(2~{S})-3-cyclohexyl-2-[[(2~{S})-4-methyl-2-[[oxidanyl(phenylmethoxycarbonylaminomethyl)phosphoryl]amino]pentanoyl]amino]propanoic acid | 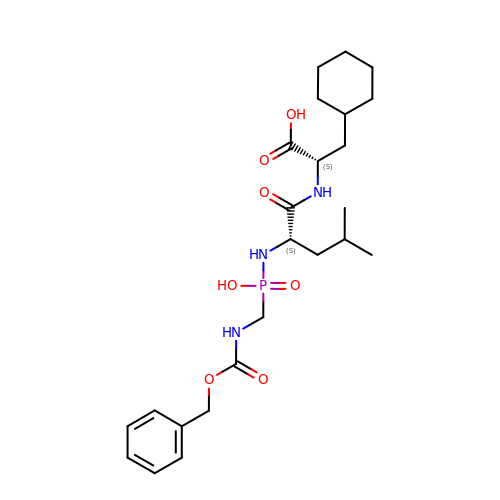C24 H38 N3 O7 P | XUMUUEQXPBWJGZ-SFTDATJTSA-N> ATFLIWPIYPKIEANEKATAVWLQNTGKTDAMVQIRVFKWNQDGLKDNYSEQSEIIPSPPVAKIKAGEKHMLRLTKSVNLPDGKEQSYRLIVDELPIRLSDGN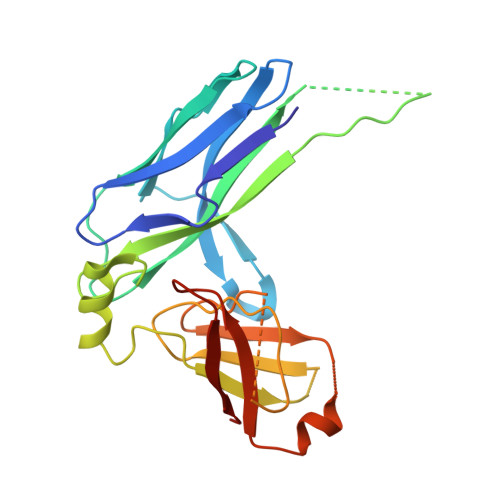EQDASKVSFQMRYSIPLFAYGKGIGSGLTEESQKLNAKNALAKPVLQWSVRNNQQGQSELYLKNNGQKFARLSALKTSKTGNDISLGKAAFGYVLSNSTVKFAIDQSTAHELAKTSKIYGVDSSGIKQELIEITKMEDPS3-{[(3,4-dichlorophenyl)carbamoyl]amino}benzoic acid | C14 H10 Cl2 N2 O3 | 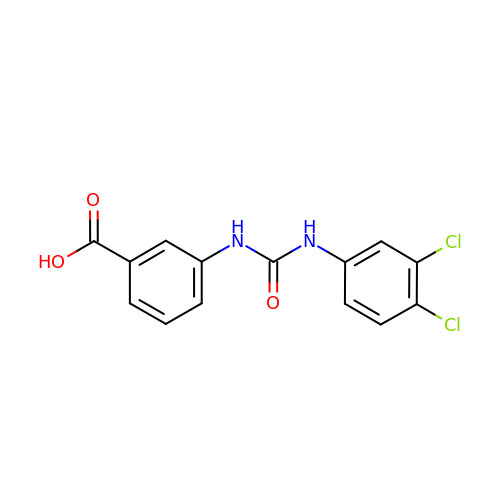RAPJIPXYCVHSNT-UHFFFAOYSA-N> MSCEIVVYPAQDSTTTNIQDISIKNYFKKYGEISHFEAFNDPNSALPLHVYLIKYASSDGKINDAAKAAFSAVRKH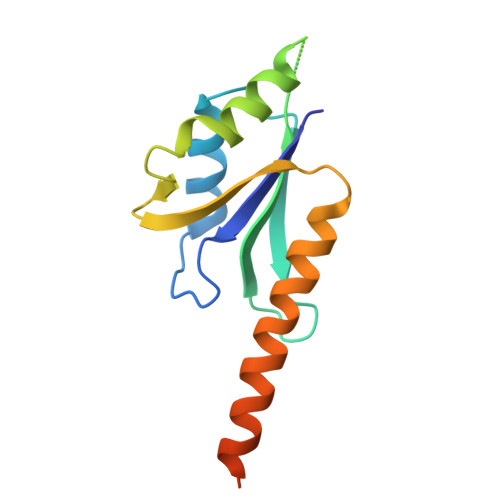ESSGCFIMGFKFEVILNKHSILNNIISKFVEINVKKLQKLQENLKKAKEKEAENHHHHHH>[2x]SMEEKLKKTNIIFVVGGPGSGKGTQCEKIVQKYGYTHLSTGDLLRSEVSSGSARGKKLSEIMEKGQLVPLETVLDMLRDAMVAKVNTSKGFLIDGYPREVQQGEEFERRIGQPTLLLYVD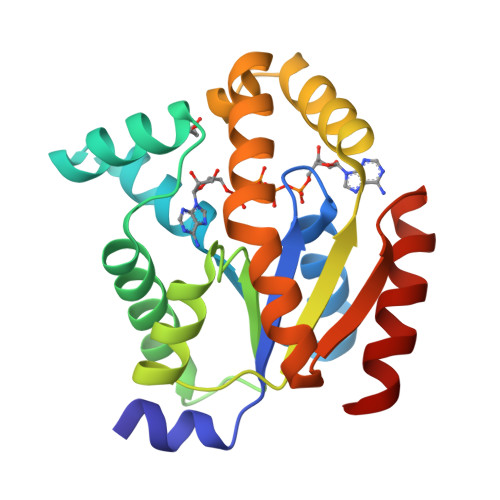AGPETMTQRLLKRGETSGRVDDNEETIKKRLETYYKATEPVIAFYEKRGIVRKVNAEGSVDSVFSQVCTHLDALLN>[3x]MKKLLPILIGLSLSGFSSLSQAENLMQVYQQARLSNPELRKSAADRDAAFEKINEARSPLLPQLGLGADYTYSNGYRDANGINSNATSASLQLTQSIFDMSKWRALTLQEKAAGIQDVTYQTDQQTLILNTATAYFNVLNAIDVLSYTQAQKEAIYRQLDQTTQRFNVGLVAITDVQNARAQYDTVLANEVTARNNLDNAVEQLRQITGNYYPELAALNVENFK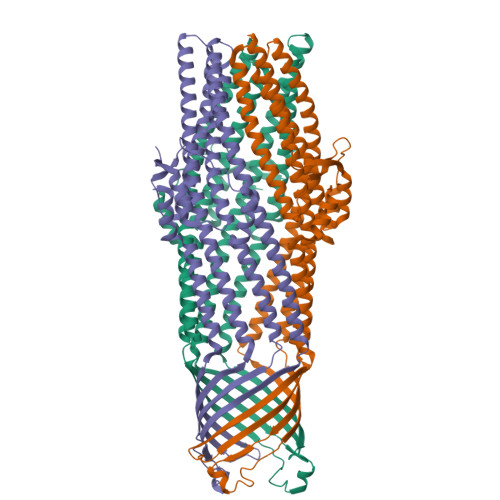TDKPQPVNALLKEAEKRNLSLLQARLSQDLAREQIRQAQDGHLPTLDLTASTGISDTSYSGSKTRGAAGTQYDDSNMGQNKVGLSFSLPIYQGGMVNSQVKQAQYNFVGASEQLESAHRSVVQTVRSSFNNINASISSINAYKQAVVSAQSSLDAMEAGYSVGTRTIVDVLDATTTLYNAKQELANARYNYLINQLNIKSALGTLNEQDLLALNNALSKPVSTNPENVAPQTPEQNAIADGYAPDSPAPVVQQTSARTTTSNGHNPFRN> ADYDLKFGMNAGTSSNEYKAAEMFAKEVKEKSQGKIEISLYPSSQLGDDRAMLKQLKDGSLDFTFAESARFQLFYPEAAVFALPYVISNYNVAQKALFDTEFGKDLIKKMDKDLGVTLLSQAYNGTRQTTSNRAINSIADMKGLKLEVPNAATNLAYAKYVGASPTPMAFSEVYLALQTNAVDGQENPLAAVQAQKFYEVQKFLAMTNHILNDQLYLVSNETYKELPEDLQKVVKDAAENAAKYHTKLFVDGEKDLVTFFEKQGVKITHPDLVPFKE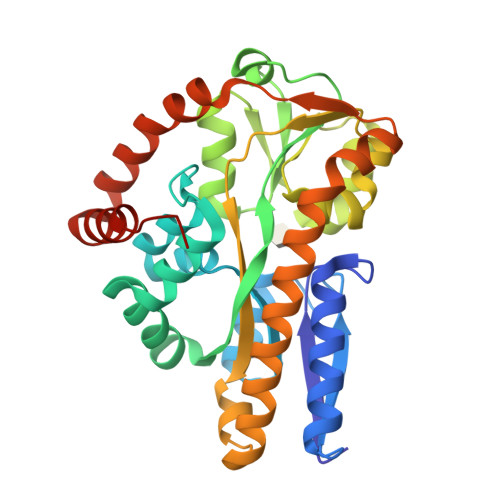SMKPYYAEFVKQTGQKGESALKQIEAINPHHHHHH(2E)-3-{5-[(2,4-diaminopyrimidin-5-yl)methyl]-2,3-dimethoxyphenyl}-1-[(1S)-1-(2-methylprop-1-en-1-yl)phthalazin-2(1H)-yl]prop-2-en-1-one | C28 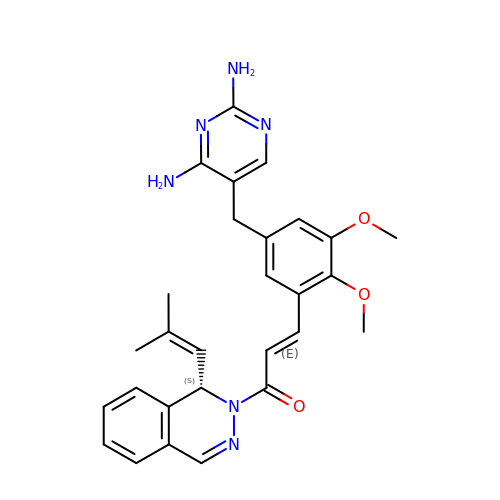H30 N6 O3 | LEKSMFBSZBQJBZ-ZUTVHTERSA-N>[2x]MSPQKSSVGVSPTLVHTLKVGFYFFLWYFFNFIFNIANKRTLNMWKYPWVLSTIQLGVGALYCTFLWVLGLRTKPNVSKKLIKALIWPSLGHTLGHAATCMSFSLVAISFTHVVKSAEPVFGAVGSALVLGEFFHPLTYLTLVPIVSGVALSAATELTFTWTGFITAMISNVAFVTRNITSKFTMVDFKNEKTLIAQNTYALITIISFFMELPFAL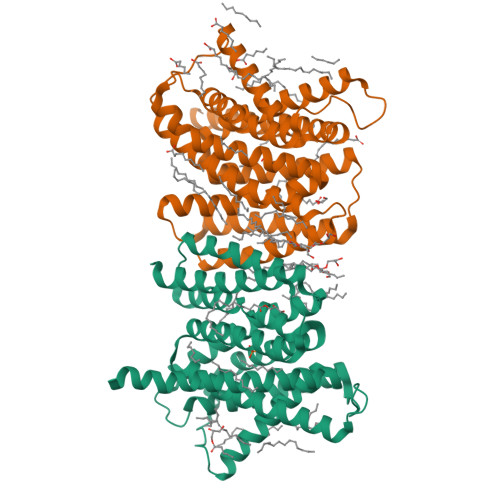LMEGFPPLVSAIAGVSKAKLFGSIMFCSLFYHLYNEVSYLCLDNVSPVSFSIGNTIKRVIIIFGSILVFRTPVTRLNFIGSTIAIIGTMLYSLAKAKLPSKREKQGTENLYFQ> MSFRPGSRGGSRGGS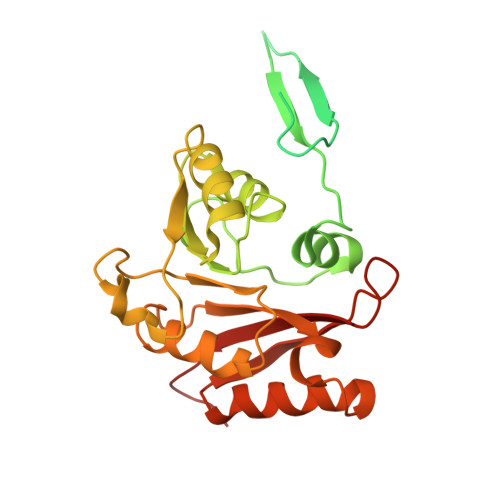RGGFGGRGGSRGGARGGSRGGFGGRGGSRGGARGGSRGGFGGRGGSRGGARGGSRGGRGGAAGGARGGAKVVIEPHRHAGVYIARGKEDLLVTKNMAPGESVYGEKRISVEEPSKEDGVPPTKVEYRVWNPFRSKLAAGIMGGLDELFIAPGKKVLYLGAASGTSVSHVSDVVGPEGVVYAVEFSHRPGRELISMAKKRPNIIPIIEDARHPQKYRMLIGMVDCVFADVAQPDQARIIALNSHMFLKDQGGVVISIKANCIDSTVDAETVFAREVQKLREERIKPLEQLTLEPYERDHCIVVGRYMRSGLKK> UCGUUGACAGGACACGAGUAACUCGUCUAUCUUCUGCAGGCUGCUUACGGUUUCGUCCGUGUUGCAGCCGAUCAUCAGCACAUCUA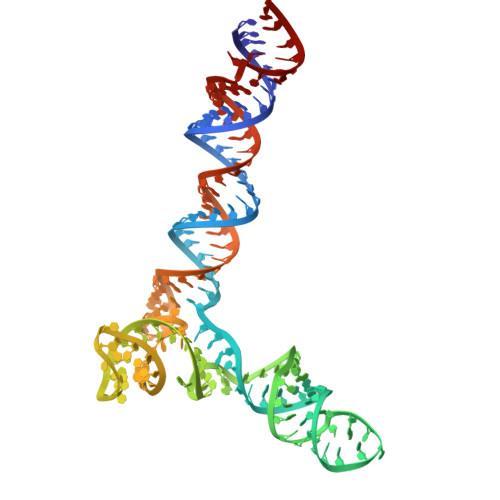GGUUUCGUCCGGGUGUGACCGAAAGGUAAGAUGGAGAGCCUUGUCCCUGGUUUCAACGA>NIYDILDKVFTMMYDGQDLTDYFLVQEVRGRSVYSIEMGKRTIAGVDGGVITTESLPARELEVDAIVFGDGTETDLRRRIEYLNFLLHRDTDV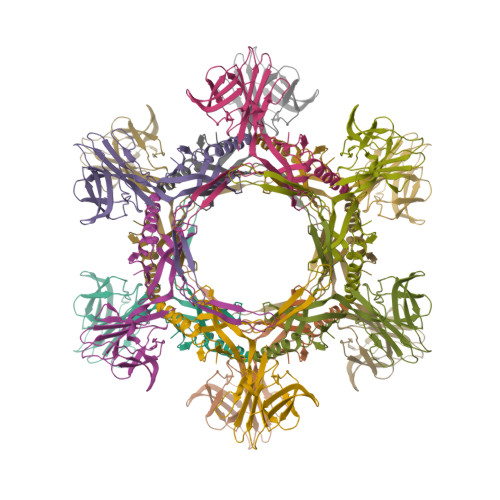PITFSDEPSRTYYGRYEFATEGDEKGGFHKVTLNFYCQDPLKYGPEVTTDVTTASTPVKNTGLAVTNPTIRCVFSTSATEYEMQLLDGSTVVKFLKVVYGFNTGDTLVIDCHERSVTLNGQDIMPALLIQSDWIQLKPQVNTYLKATQPSTIVFTEKFL[3x]> AFTKRGASSYVRETLPVLTRTVVPADNSCLFTSVYYVVEGGVLNPACAPEMRRLIAQIVASDPDFYSEAILGKTNQEYCDWIKRDDTWGGAIEISILSKFYQCEICVVDTQTVRIDRFGEDAGYTKRVLLIYDGIHYDPLQRNFPDPDTPPLTIFSSNDDIVLVQALELADEARRRRQFTDVN

Sixteen ovarian tumor (OTU) family deubiquitinases (DUBs) exist in humans, and most members regulate cell-signaling cascades. Biochemical analysis and five crystal structures of OTU DUBs with or without Ub substrates reveal four mechanisms of linkage specificity. Mechanistic and structural studies of three closely related, unstudied OTUs with distinct cleavage profiles revealed four mechanisms for achieving linkage specificity, namely (1) the use of additional Ub-binding domains (UBDs), (2) specific recognition of a ubiquitinated sequence, (3) the use of a conserved S1’ Ub-binding site on the OTU domain itself, and (4) the use of an S2 site enabling DUBs to bind longer chains in a linkage-specific manner. We selected three members of the OTUD family for additional investigation: the unstudied Lys63-specific OTUD1, the cdc48/p97 interactor OTUD2 that cleaves atypical linkages (Lys11, Lys27, Lys29, and Lys33), and OTUD3, another unstudied DUB with activity against Lys6- and Lys11-linked diUb.

To understand the specificity of OTUD domains at the molecular level, we determined high-resolution crystal structures of OTUD1 (aa 287–437, 2.1 Å), OTUD2 (aa 132–314, 1.5 Å), and OTUD3 (aa 52–209, 1.55 Å). The catalytic domains are structurally similar to each other and to OTUD5 (Huang et al., 2012) and S. cerevisiae Otu1 (yOtu1) (Messick et al., 2008), root-mean-square deviations (rmsds) being from 0.6–1.0 Å. Catalytic triads are in competent conformations, as observed for pOTUD5 in complex with a Ub suicide probe (Huang et al., 2012). In OTUD1, OTUD2, and OTUD3, the corresponding secondary structure elements are present with or without Ub bound, and there are no large-scale conformational changes in OTUD2 upon Ub binding. Full-length OTUD2 cleaved Lys11-, Lys27-, Lys29-, and Lys33-linked diUb. Removal of the N-terminal UBX-like domain did not affect OTUD2 specificity, but deletion of the C-terminal ZnF domain or point mutations in zinc-binding residues significantly reduced activity toward Lys27-, Lys29-, and Lys33-linked diUb without affecting Lys11 activity. Hence, the ZnF domain in OTUD2 enabled a Lys11-specific catalytic core domain to cleave three additional linkage types. Along with these loops, the N-terminal helix in the OTUD1 and OTUD3 catalytic domain and the structurally equivalent C-terminal helix of the OTUD2 catalytic domain form the putative S1’ site that binds the proximal Ub. S. cerevisiae encode only two OTU DUBs, yOtu1 and yOtu2. yOtu1 and D. melanogaster (dm) Otu1 are orthologs of human OTUD2 (38% and 53% identical in OTU domain, respectively), and OTUD2 and yOtu1 both bind cdc48/p97 and are involved in endoplasmic-reticulum-associated protein degradation (Ernst et al., 2009; Rumpf and Jentsch, 2006).>GSPEFSLDVRQEELGAVVDKEMAATSAAIEDAVRRIEDMMNQARHASSGVKLEVNERILNSCTDLMKAIRLLVTTSTSLQKEIVESGRGAATQQEFYAKNSRWTEGLISASKAVGWGATQLVEAADKVVLHTGKYEELIVCSHEIAASTAQLVAASKVKANKHSPHLSRLQECSRTVNERAANVVASTKSGQEQIEDRDTMDFSGL[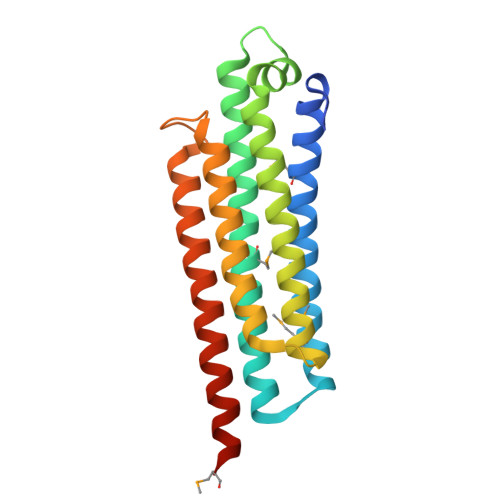8x]>[4x]GHMKTVVFAYHDMGCLGIEALLAAGYEISAIFTHTDNPGEKAFYGSVARLAAERGIPVYAPDNVNHPLWVERIAQLSPDVIFSFYYRHLIYDEILQLAPAGAFNLHGSLLPKYRGRAPLNWVLV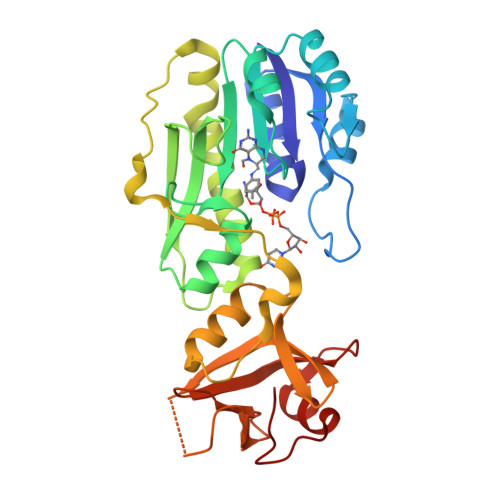NGETETGVTLHRMVKRADAGAIVAQLRIAIAPDDIAITLHHKLCHAARQLLEQTLPAIKHGNILEIAQRENEATCFGRRTPDDSFLEWHKPASVLHNMVRAVADPWPGAFSYVGNQKFTVWSSRVHPHASKAQPGSVISVAPLLIACGDGALEIVTGQAGDGITMQGSQLAQTLGLVQGSRLNS> MTIRHHVSDALLTAYAAGTLSEAFSLVVATHLSLCDECRARAGALDAVGGSLMEETAPVALSEGSLASVMAQLDRQIQRPAPARRADPRAPAPLAD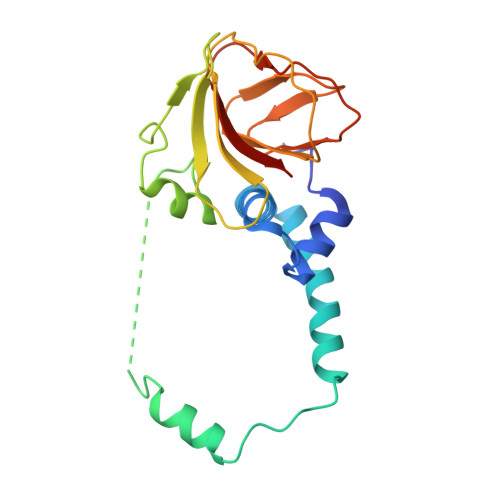YVGRRLEDVRWRTLGGGVRQAILPTGGEAIARLLWIPGGQAVPDHGHRGLELTLVLQGAFRDETDRFGAGDIEIADQELEHTPVAERGLDCICLAATDA> MKAYMFPGQGSQAKGMGRALFDAFPALTARADGVLGYSIRALCQDDPDQRLSQTQFTQPALYVVNALSYLKRREEEAPPDFLAGHSLGEFSALFAAGVFDFETGLALVKKRGELMGDARGGGMAAVIGLDEERVRELLDQNGATAVDIANLNSPSQVVISGAKDEIARLQVPFEAAGAKKYTVLRVSAAFHSRFMRPAMVEFGRFLEGYDFAPPKIPVISNVTARPCKADGIRAALSEQIAS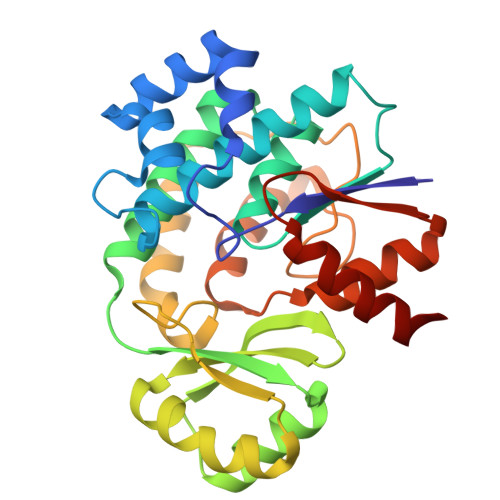PVRWCESIRYLMGRGVEEFVECGHGIVLTGLYAQIRRDAQ> MTEQQKLTFTALQQRLDSLMLRDRLRFSRRLHGVKKVKNPDAQQAIFQEMAKEIDQAAGKVLLREAARPEITYPDNLPVSQKKQDILEAIRDHQVVIVAGETGSGKTTQLPKICMELGRGIKGLIGHTQPRRLAARTVANRI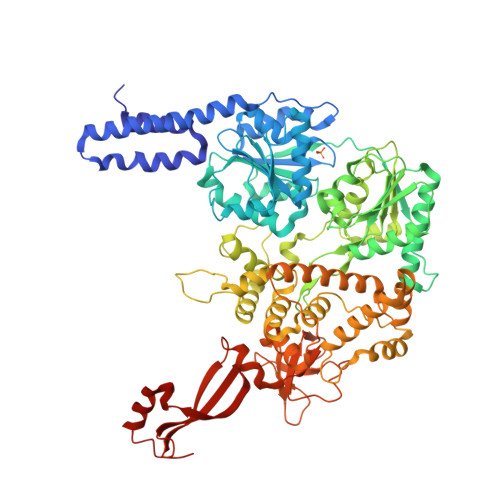AEELKTEPGGCIGYKVRFSNHVSDNTMVKLMTDGILLAEIQQDRLLMQYDTIIIDEAHERSLNIDFLLGYLKELLPRRPDLKIIITSATIDPERFSRHFNNAPIIEVSGRTYPVEVRYRPIVEEADDTERDQLQAIFDAVDELSQESPGDILIFMSGEREIRDTADALNKLNLRHTEILPLYARLSNSEQNRVFQSHSGRRIVLATNVAETSLTVPGIKYVIDPGTARISRYSYRTKVQRLPIEPISQASANQRKGRCGRVSEGICIRLYSEDDFLSRPEFTDPEILRTNLASVILQMTALGLGDIAAFPFVEAPDKRNIQDGVRLLEELGAITTDEQASAYKLTPLGRQLSQLPVDPRLARMVLEAQKHGCVREAMIITSALSIQDPRERPMDKQQASDEKHRRFHDKESDFLAFVNLWNYLGEQQKALSSNAFRRLCRTDYLNYLRVREWQDIYTQLRQVVKELGIPVNSEPAEYREIHIALLTGLLSHIGMKDADKQEYTGARNARFSIFPGSGLFKKPPKWVMVAELVETSRLWGRIAARIDPEWVEPVAQHLIKRTYSEPHWERAQGAVMATEKVTVYGLPIVAARKVNYSQIDPALCRELFIRHALVEGD2-methylpyrimidin-4-amine 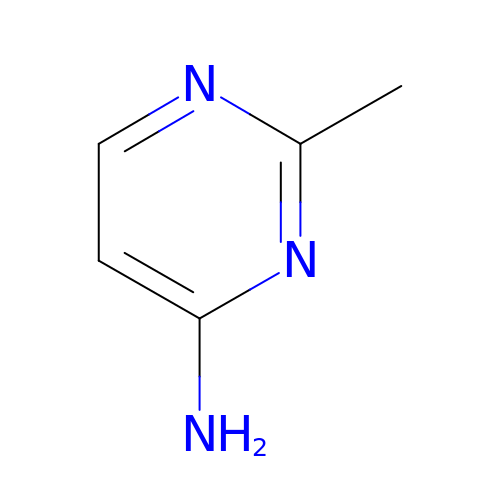| C5 H7 N3 | GKVDLTTVBNOGNJ-UHFFFAOYSA-N> MGSDKIHHHHHHM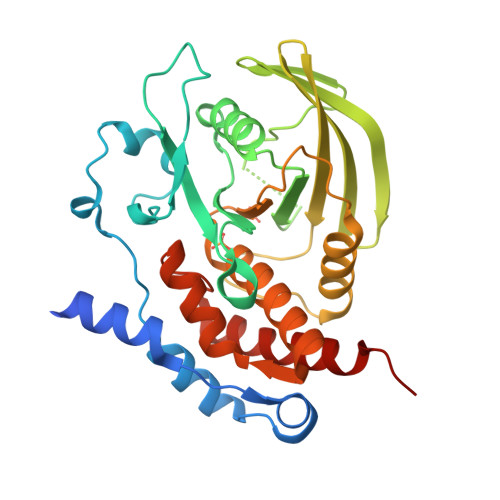NTPREVTLHFLRTAGHPLTRWALQRQPPSPKQLEEEFLKIPSNFVSPEDLDIPGHASKDRYKTILPNPQSRVCLGRAQSQEDGDYINANYIRGYDGKEKVYIATQGPMPNTVSDFWEMVWQEEVSLIVMLTQLREGKEKCVHYWPTEEETYGPFQIRIQDMKECPEYTVRQLTIQYQEERRSVKHILFSAWPAHQTPESAGPLLRLVAEVEESPETAAHPGPIVVHSSAGIGRTGCFIATRIGCQQLKARGEVDILGIVCQLRLDRGGMIATAEQYQFLHHTLALYAGQLPEEPSP2-methyl-5-(1-methylethyl)cyclohexa-2,5-diene-1,4-dione 1-oxime | 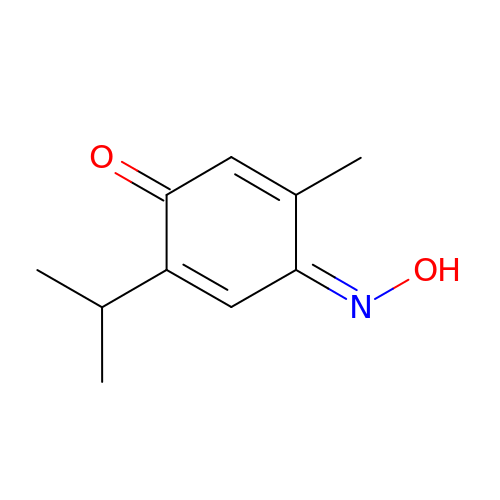C10 H13 N O2 | LFDOSYRMCCGDBT-PKNBQFBNSA-N>MKEHRHMTEKSPHSAFGDGAKAYDVPAFGLQIHTVEHGSGAPIVFLHGNPTSSYLWRHIFRRLHGHGRLLAVDLIGYGQSSKPDIEYTLENQQRYVDAWFDALDLRNVTLVLQDWGAAFGLNWASRNPDRVRAVAFFEPVLRNIDSVDLSPEFVTRRAKLRQPGEGEIFVQQENRFLTELFPWFFLTPLAPEDLRQYQTPFPTPHSRKAILAGPRNLPVDGEPASTVAFLEQAVNWLNTSDTPKLLLTFKPGFLLTDAILKWSQVTIRNLEIEAAGAGIHFV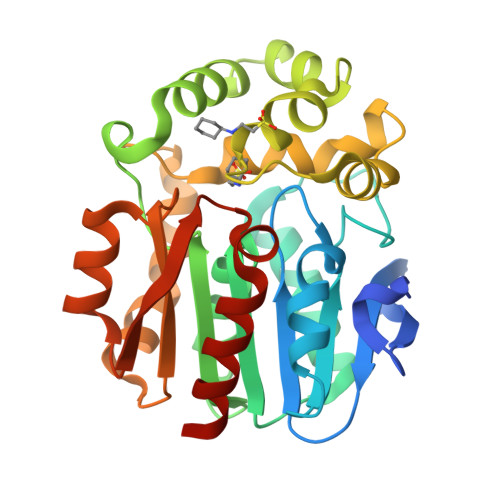QEEQPETIARLLDAWLTRIAGN[2x]N-{[4-CHLORO-3-(TRIFLUOROMETHYL)PHENYL]SULFONYL}-L-TRYPTOPHAN | C18 H14 Cl F3 N2 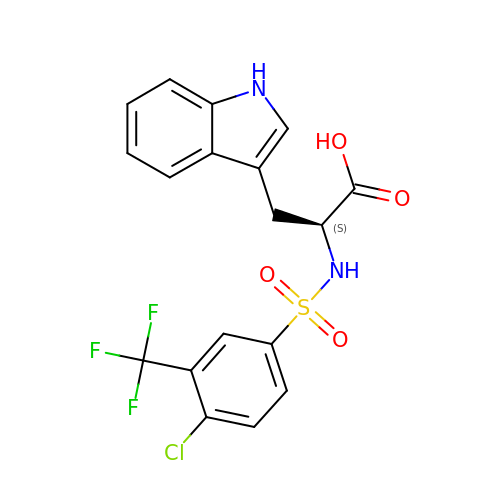O4 S | YOZOZANENKPWEP-INIZCTEOSA-N>[4x]GGADQKGPVFLKEPTNRIDFSNSTGAEIECKASGNPMPEIIWIRSDGTAVGDVPGLRQISSDGKLVFPPFRAEDYRQEVHAQVYACLARNQFGSIISRDVHVRAVVNQFYEAEIMTEYV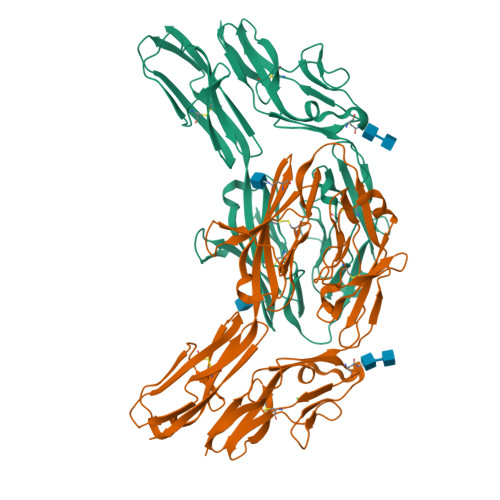IRGNAAVLKCSIPSFVADFVRVESWIDDEGNVLSFSDNYDGKYLVLPSGELHIREVGPEDGYKSYQCRTKHRLTGETRLSATKGRLVITEPVGSKAPTFATASKISSLLGSSSSDIVLLCQAQAFPVPYTRWYKFIEGTTRKQAVVLNDRVKQVSGTLIIKDAVVEDSGKYLCVVNNSVGGESVETVLTVTAPLSAKIDPPTQTVDFGRPAVFTCQYTGNPIKTVSWMKDGKAIGHSEPVLRIESVKKEDKGMYQCFVRNDQESAEASAELKLGG> MARPFKFPRSYAALLADWPVVVLGMCTLLIVVCALVGVLVPELPDFSDPLLGFEPRGTTIGQRLVTWNNMMRNTGYKATLANYPYKYAEEQARSHRDDRWSDDHHERERREVDWNFQKDSFFCDVPSDGYSRVVFASAGGETLWNLPAIKSMCDVDNSRIRSHPQFSDLCQRTTAVSCCPSWTLGNYIAILNNRSSCQKIVERDVSHTLKLLRTCAKHYQNGTLGPDCWDKAARRKDQLKCTNVPRKCTKYNAVYQILHYLVDKDFMTPKTADYAVPALKYSMLFSPTEKGESMMNIYLDNFENWNSSDGITTVTGIEFGIKHSLFQDYL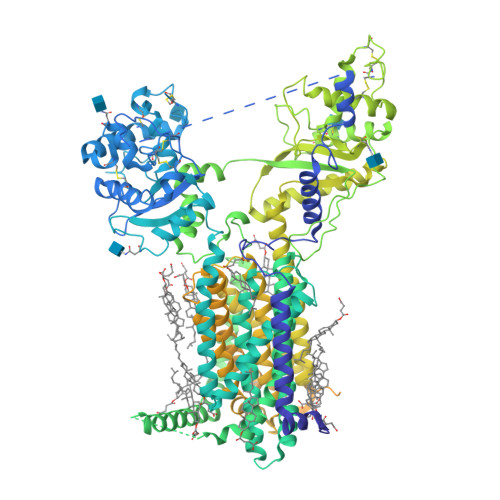LMDTVYPAIAIAIVLLIMCVYTKSMFITLMTMFAIISSLIVSYFLYRVVFNFEFFPFMNLTALIILVGIGANNAFVLCDVWNYTKFDKPRAETSEAVSVTLQHAALSMFVTSFTTAAAFYANYVSNITAIRCFGVYAGTAILVNYVLMVTWLPAVIVLHERYLLNIFTCFRKPQPQAYDKSCWAVLCQKCRRVLFAVSEASRIFFEKVLPCIVIKFRYLWLIWFLALTVGGAYIVCVNPKMKLPSLELSEFQVFRSSHPFERYDAEFKKLFMFERVHHGEELHMPITVIWGVSPEDSGDPLNPKSKGELTLDSTFNIASPASQAWILHFCQKLRNQTFFHQTEQQDFTSCFIETFKQWMENQDCDEPALYPCCSHCSFPYKQEVFELCIKKAIMELDRSTGYHLNNKTPGPRFDINDTIRAVVLEFQSTFLFTLAYEKMQQFYKEVDSWISHELSSAPEGLSRGWFVSNLEFYDLQDSLSDGTLIAMGLSVAVAFSVMLLTTWNIIISLYAIVSIAGTIFVTVGSLVLLGWELNVLESVTISVAVGLSVNFAVHYGVAYRLAPDPDREGKVIFSLSRMGSAIAMAALTTFVAGAMMMPSTVLAYTQLGTFMMLVMCVSWAFATFFFQCLCRCLGPQGTCGQIPFPTKLQCSPFSHTLSARPGDRGPSKTHAASAYSVDARGQKSQLEHEFYELQPLASHSCTSSEKTTYEEPHTCSEFFNGQAKNLRMPVPAAYSSELTKSPSSEPGSALLQSCLEQDTVCHFSLNPRCNCRDAYTHLQYGLPEIHCQQMGDSLCHKCASTAGGFVQIQSSVAPLKASHQAAEGLLHPAQHMLPPGMQNSRPRNFFLHSVQHFQAQENLGRTSTHSTDERLPRTAELSPPPSDSRSTESFQRACCHPENNQRRLCKSRDPGDTEGSGGTKSKVSGLPNQTDKEEKQVEPSLLQTDETVNSEHLNHNESNFTFSHLPGEAGCRSCPNSPQSCRSIMRSKCGTEDCQTPNLEANVPAVPTHSDLSGESLLIKTL> GKAFDDGAFTGIREINLSYNKETAIGDFQVVYDLNGSPYVGQNHVSFITGFTPVKISLDF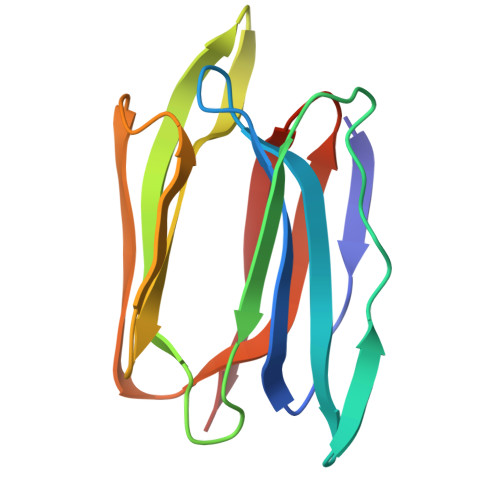PSEYIMEVSGYTGNVSGYVVVRSLTFKTNKKTYGPYGVTSGTPFNLPIENGLIVGFKGSIGYWLDYFSMYLSL> MDSSPNEFLNKVIGKKVLIRLSSGVDYKGILS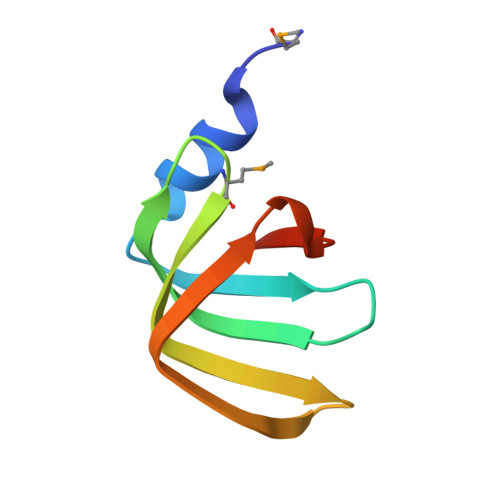CLDGYMNLALERTEEYVNGKKTNVYGDAFIRGNNVLYVSALDD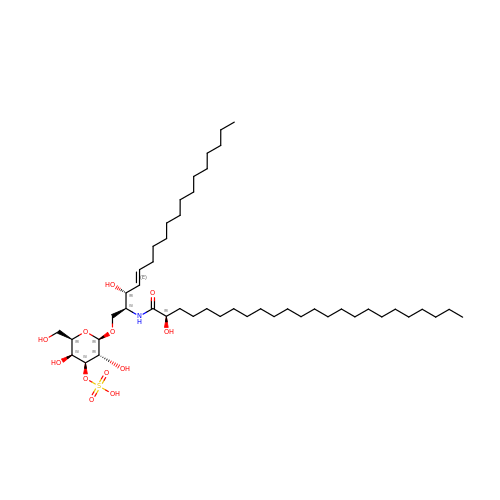SULFOGALACTOCERAMIDE | C48 H93 N O12 S | QTTLKKFUOJQIRB-JOLIRYOJSA-N(2~{S})-6-azanyl-2-[[(2~{S})-4-methyl-2-[[oxidanyl(phenylmethoxycarbonylaminomethyl)phosphoryl]amino]pentanoyl]amino]hexanoic acid | C21 H35 N4 O7 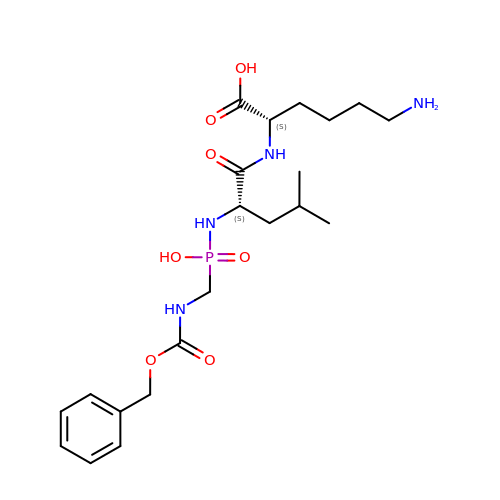P | QNYUXDGTIPHQBZ-ROUUACIJSA-N> MSNWVMQEENKQGNLTPLFEELLQQCPPGGQNKTAHMVSAYQLAQGNWMPTSCHVFMGTISARRTKTHPYEAYVKLRELVEEHKMKTLCPGSSLGKHNDWIIGKIKYQGNLRTKHMLNPGKVAEQLCREGHRHNVYNKTIGSVMTATGIRLEKLPVVRAQTDTTNFHQAIRDKIDKEENLQTPGLHKKLMEVFNALKRPELESSYDAVEWEELERGINRKGAAGFFERKNIGEILDSEKNKVEEIIDNLKKGRNIKYYETAIPKNEKRDVNDDWTAGDFVDEKKPRVIQYPEAKTRLAITKVMYKWVKQKPVVIPGYEGKTPLFQIFDKVKKEWDQFQNPVAVSFDTKAWDTQVTTKDLELIKDIQKYYFKKKWHKFIDTLTMHMTEVPVICADGEVYIRKGQRGSGQPDTSAGNSMLNVLTMVYAFCEATGVPYKSFDRVAKIHVCGDDGFLITERALGEKFASKGVQILYEAGKPQKITEGDKMKVAYQFDDIEFCSHTPIQVRWSDNTSSYMPGRNTTTILAKMATRLDSSGERGTIAYEKAVAFSFLLMYSWNPLIRRICLLVLSTELQVKPGKSTTYYYEGDPISAYKEVIGHNLFDLKRTSFEKLAKLNLSMSVLGAWTRHTSKRLLQDCVNMGVKEGNWLVNADRLVSSKTGNRYIPGEGHTLQGRHYEELVLARKQINNFQGADRYNGSSSHHHHHH

Compared to the RdRPs of other Flaviviridae representatives such as the NS5 of the Japanese encephalitis virus (JEV) and dengue virus (DENV) in the Flavivirus genus and the NS5B of the hepatitis C virus (HCV) of the Hepacivirus genus, the pestivirus NS5B contains a unique ∼90-residue N-terminal domain (NTD) that does not have notable sequence homology to any other viral or host proteins. The global conformation of our CSFV NS5B structures is consistent with the recently reported CSFV structure with an RMSD value of 0.9 Å (95% coverage) between the reported structure and our representative C-682 structure. These structures together reveal that the NTD adopts a globular α/β fold with an α-β-α-β-β-α pattern. The NTD interacts with the palm of the RdRP core intra-molecularly with a mixture of hydrophobic and hydrogen bonding interactions. Collectively, these biochemical data indicated that the RNA synthesis fidelity of CSFV NS5B is fine-tuned by its NTD through the intra-molecular interactions with the RdRP palm.

In order to investigate the function of the NTD of CSFV NS5B, we first made an NS5B construct comprising residues 1–694 with only the C-terminal hydrophobic region removed. For description purpose, we herein named this construct as the wild-type (WT). This construct was soluble and capable in GG dinucleotide driven RNA synthesis using a template RNA sequence derived from the RdRP assays established in the HCV NS5B and the JEV NS5 (53,58). The structure of the WT was solved at 2.5 Å resolution in space group P43212 by molecular replacement using a BVDV NS5B structure comprising residues 91–672 as the search model. The structures of the C-682 and C-672 were solved at 2.1 and 2.3 Å resolution, respectively, in the same crystal form by molecular replacement using the structure of the WT as the search model. These three structures, each containing one NS5B molecule in the crystallographic asymmetric unit, are highly similar with root mean square deviation (RMSD) values of 0.4–0.6 Å between the WT and two C-terminal truncation mutants for all superimposable α-carbon atoms with 99% coverage of the resolved residues in the structure of the WT. In the structures of the WT and C-682, residues beyond 672 are disordered. Although this conformation is likely not compatible with de novo initiation, normal activity of the WT and C-682 observed in the polymerase assays suggests that the canonical conformation also exist in solution and may be in equilibrium with the observed bent conformation observed in the crystal structures. In a time course reaction, WT NS5B exhibited low level of misincorporation with the mismatch fraction gradually increasing over time and reached about 0.25 at the 180-min time point. Lying in the heart of this NTD–RdRP interface, are two adjacent RdRP residues Y471 and E472.> VVRREWLEEAQENKIYFLLQVDYDGKKGKAVCKLFDKETQKIYALYDNTGHKPYFLVDLEPDKVGKIPKIVRDPSFDHIETVSKIDPYTWNKFKLTKIVVRDPLAVRRLRNDVPKAYEAHIKYFNNYMYDIGLIPGMPYVVKNGKLESVYLSLDEKDVEEIKKAFADSDEMTRQMAVDWLPIFETEIPKIKRVAIDIEVYTPVKGRIPDSQKAEFPIISIALAGSDGLKKVLVLNRNDVNEGSVKLDGISVERFNTEYELLGRFFDILLEYPIVLTFNGDDFDLPYIYFRALKLGYFPEEIPIDVAGKDEAKYLAGLHIDLYKFFFNKAVRNYAFEGKYNEYNLDAVAKALLGTSKVKVDTLISFLDVEKLIEYNFRDAEITLQLTTFNNDLTMKLIVLFSRISRLGIEELTRTEISTWVKNLYYWEHRKRNWLIPLKEEILAKSSNIRTSALIKGKGYKGAVVIDPPAGIFFNITVLDFASLYPSIIRTWNLSYETVDIQQCKKPYEVKDETGEVLHIVCMDRPGITAVITGLLRDFRVKIYKKKAKNPNNSEEQKLLYDVVQRAMKVF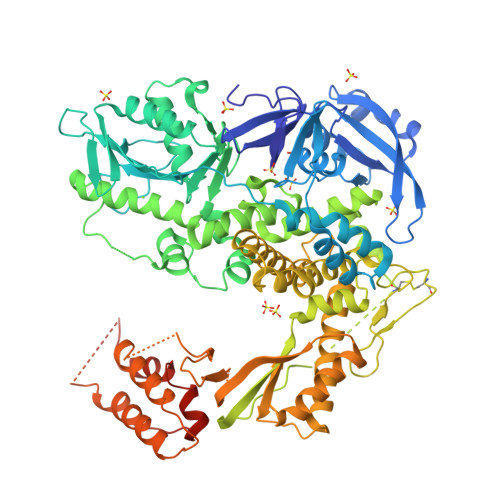INATYGVFGAETFPLYAPRVAESVTALGRYVITSTVKKAREEGLTVLYGDTDSLFLLNPPKNSLENIIKWVKTTFNLDLEVDKTYKFVAFSGLKKNYFGVYQDGKVDIKGMLVKKRNTPEFVKKVFNEVKELMISINSPNDVKEIKRKIVDVVKGSYEKLKNKGYNLDELAFKVMLSKPLDAYKKNTPQHVKAALQLRPFGVNVLPRDIIYYVKVRSKDGVKPVQLAKVTEIDAEKYLEALRSTFEQILRAFGVSWDEIAATMSIDSFFSYPSKGNS>SSSSTASASAKKIIVKHVTVIGGGLMGAGIAQVAAATGHTVVLVDQTEDILAK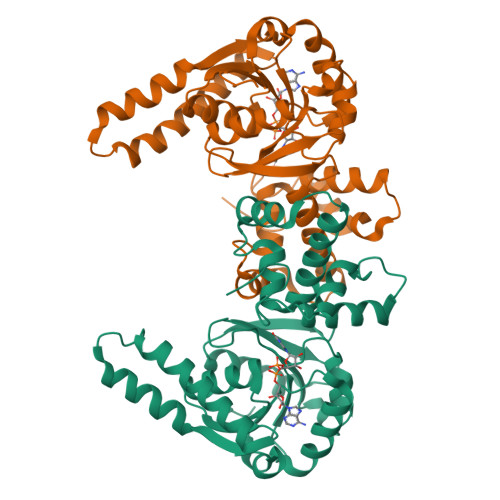SKKGIEESLRKVAKKKFAENPKAGDEFVEKTLSTIATSTDAASVVHSTDLVVEAIVENLKVKNELFKRLDKFAAEHTIFASNTASLQITSIANATTRQDRFAGLHFFNPVPVMKLVEVIKTPMTSQKTFESLVDFSKALGKHPVSCKDTPGFIVNRLLVPYLMEAIRLYERGDASKEDIDTAMKLGAGYPMGPFELLDYVGLDTTKFIVDGWHEMDAENPLHQPSPSLNKLVAENKFGKKTGEGFYKYK[2x]>[180x]MEIYEGKLTAEGLRFGIVASRFNHALVDRLVEGAIDCIVRHGGREEDITLVRVPGSWEIPVAAGELARKEDIDAVIAIGVLIEGAEPHFDYIASEVSKGLANLSLELRKPITFGVITADELEEAIERAGTKHGNKGWEAALSAIEMANLFKSLRLEHHHHH

One highly versatile encapsulation system has been engineered from the capsid-forming enzyme lumazine synthase from the hyperthermophilic bacterium Aquifex aeolicus. In nature, these structures encapsulate riboflavin synthase, an enzyme that converts lumazine to riboflavin. In the structures of the AaLS variants, the pentamer is the common and exclusive building block for all assemblies. Here, we elucidate the structures of the AaLS protein containers by native mass spectrometry (MS) and cryo-EM single-particle reconstruction techniques.

To bind unrelated guests, we mutated four residues that project into the lumen of the capsid to negatively charged glutamates. The resulting variant, called AaLS-neg, encapsulates proteins with complementary positive charges. For AaLS-neg, a similarly well-resolved spectrum was obtained that corresponds to a 180-mer (measured mass of 3.02 MDa, theoretical mass of 3.01 MDa) in agreement with the predicted icosohedral T=3 structure. In the case of AaLS-neg, contrary to expectations for a conventional T=3 state21, imposing icosahedral symmetry during reconstruction did not result in interpretable density. By assuming tetrahedral symmetry, however, we obtained an initial reconstruction that was consistent with the distinct patterns of the 2D class-averages. The secondary structure elements of each subunit could be unambiguously assigned in the final EM density map refined to 5.4 Å resolution from 26,769 particles. The 180 subunits of AaLS-neg, organized as 36 pentameric building blocks, form a novel 29-nm hollow tetrahedral cage with large, keyhole-shaped pores in the shell. Superposition of AaLS-neg pentamers onto AaLS-wt pentamers revealed that the individual subunits of the engineered variant are slightly tilted outwards from the five-fold rotational symmetry axes (Cα RMSDs of 2.1–2.3 Å). This conformational change, which modifies the wedge-like shape of the pentamer, is likely the result of electrostatic repulsion between the anionic residues that were introduced on the lumenal surface. AaLS-neg and AaLS-13 possess 12 and 30 such openings, respectively, yet maintain high thermal stability.> ALGSVTDRHAAEYNMRHKNRGMALIFNHEHFEVPTLKSRAGTNVDCENLTRVLKQLDFEVTVYKDCRYKDILRTIEYAASQNHSDSDCILVAILSHGEMGYIYAKDTQYKLDNIWSFFTA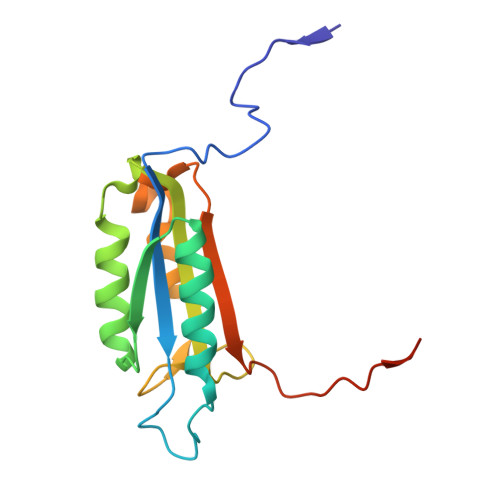NHCPSLAGKPKLFFIQACQGDRLDGGVTMQRSQTETD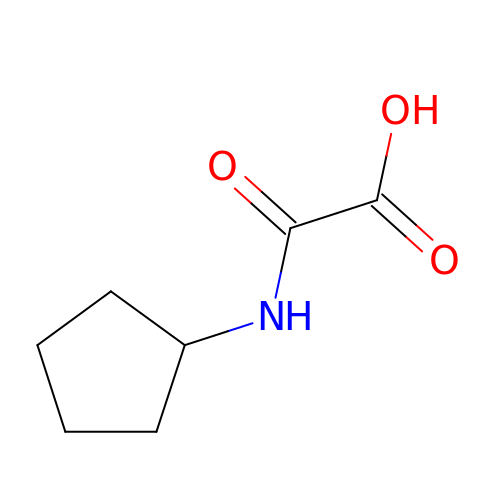(cyclopentylamino)(oxo)acetic acid | C7 H11 N O3 | XYYFQOQNHIZVBG-UHFFFAOYSA-N> GAMGSSRKSKAELQSEERKRIDELIESGKEEGMKIDLIDGKGRGVIATKQFSRGDFVVEYHGDLIEITDAKKREALYAQDPSTGCYMYYFQYLSKTYCVDATRETNRLGRLINHSKCGNCQTKLHDIDGVPHLILIAS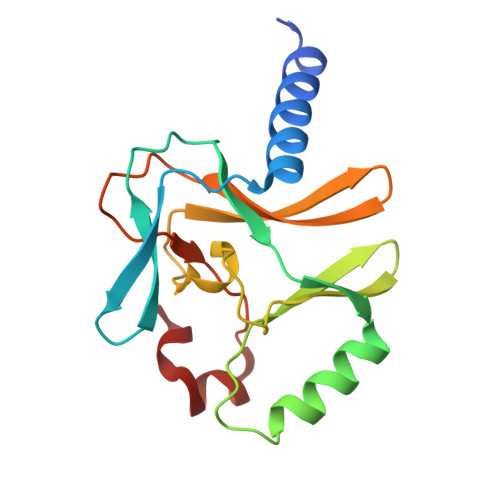RDIAAGEELLYDYGDRSKASIEAHPWLKH The coat proteins (CPs) of single-stranded RNA bacteriophages (ssRNA phages) directly assemble around the genomic RNA (gRNA) to form a near-icosahedral capsid with a single maturation protein (Mat) that binds the gRNA and interacts with the retractile pilus during infection of the host. The canonical ssRNA phage Qβ has a genomic RNA (gRNA) of 4217 nucleotides, from the 5′ to the 3′ end, encoding the maturation protein (Mat); the major coat protein (CP); the minor capsid protein A1, which is a read-through extension caused by a leaky stop codon for the major CP; and the β-subunit of the RNA-dependent RNA replicase (Rep). Like many other viruses, the CPs of ssRNA phages can also assemble into virus-like particles (VLPs), which are not infectious. Through a native infection without engineering the amino acid sequences, we found that Qβ CP can form diverse VLP capsids, including the T = 3 icosahedral, T = 4 icosahedral, prolate, oblate, and a small prolate form elongated along the 3-fold axis.

Besides the 5-fold non-icosahedral capsids, Qβ can also form a small prolate VLP elongated along the 3-fold axis, which is a new conformation of the virus capsid. In the elongated face, different from the 5-fold capsids having the same triangulation number, the 3-fold small prolate consists of two different triangulation numbers, Q1 = 2 and Q2 = 3. Moreover, the triangulation number of the two caps in the small prolate is T = 1, which means that Qβ has the potential to form a T = 1 icosahedral VLP. However, we did not find the T = 1 capsids in this study. The elongated faces of the small prolate consist of two triangulation numbers, Q1 = 2 and Q2 = 3. For the oblate and small prolate VLPs, there are two types of hexamers in each form. The “over arched” type, which provides more curvature with a θ angle of ~130°, includes hexamers from the oblate and small prolate VLPs. When produced from an infection event, and purified via size-exclusion chromatography, the population of the oblate and the small prolate forms are around 21% and 3%, respectively. When over-expressing the gene containing only the cp and read-through (referred to as A1) fraction of the Qβ genome from a plasmid, the percentage of the oblate and small prolate forms increase further to 35% and 12%, respectively. Two forms of these VLPs, namely, the oblate and the D3 symmetrical small-prolate forms, have not been observed before.

>[22x]MAKLETVTLGNIGKDGKQTLVLNPRGVNPTNGVASLSQAGAVPALEKRVTVSVSQPSRNRKNYKVQVKIQNPTACTANGSCDPSVTRQAYADVTFSFTQYSTDEERAFVRTELAALLASPLLIDAIDQLNPAY> MSYYHHHHHHLESTSLYKKAGLVQRITIAPQGPEFSRFVMGYWRLMDWNMSARQLVSFIEEHLDLGVTTVDHADIYGG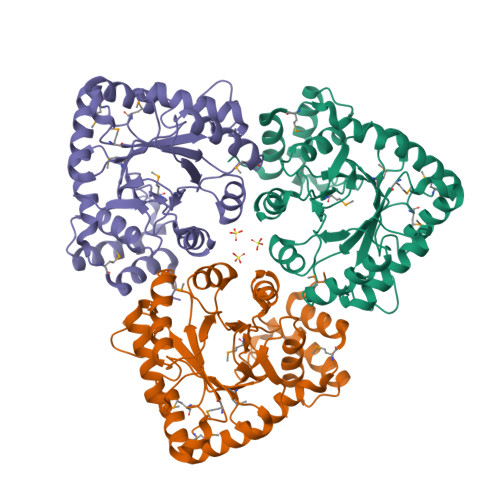YQCEAAFGEALKLAPHLRERMEIVSKCGIATTAREENVIGHYITDRDHIIKSAEQSLINLATDHLDLLLIHRPDPLMDADEVADAFKHLHQSGKVRHFGVSNFTPAQFALLQSRLPFTLATNQVEISPVHQPLLLDGTLDQLQQLRVRPMAWSCLGGGRLFNDDYFQPLRDELAVVAEELNAGSIEQVVNAWVLRLPSQPLPIIGSGKIERVRAAVEAETLKMTRQQWFRIRKAALGYDVP>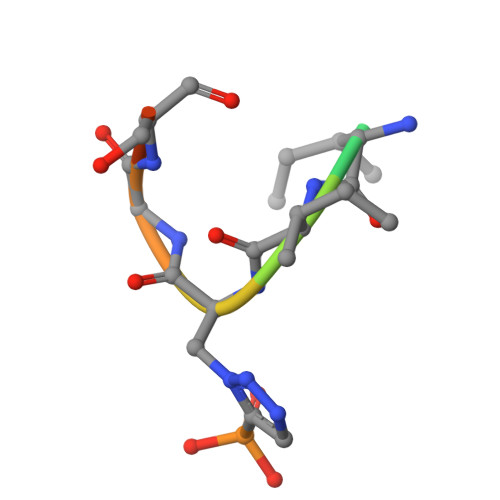 RNIIXGSDS>MKVGIVGSGMVGSATAYALALLGVAREVVLVDLDRKLAQAHAEDILHATPFAHPVWVRAGSYGDLEGARAVVLAAGVAQRPGETRLQLLDRNAQVFAQVVPR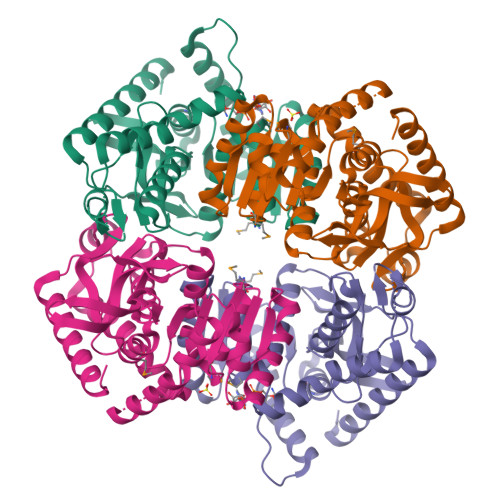VLEAAPEAVLLVATNPVDVMTQVAYRLSGLPPGRVVGSGTILDTARFRALLAEYLRVAPQSVHAYVLGEHGDSEVLVWSSAQVGGVPLLEFAEARGRALSPEDRARIDEGVRRAAYRIIEGKGATYYGIGAGLARLVRAILTDEKGVYTVSAFTPEVEGVLEVSLSLPRILGAGGVEGTVYPSLSPEEREALRRSAEILKEAAFALGF[8x]> SRVLLALHDRAPQLKISDDRLTVVGEKGYSMVRASHGVRKGAWYFEITVDEMPPDTAARLGWSQPLGNLQAPLGYDKFSYSWRSKKGTKFHQSIGKHYSSGYGQGDVLGFYINLPEDISGRGSEIIFYKNGVNQGVAYKDIFEGVYFPAIS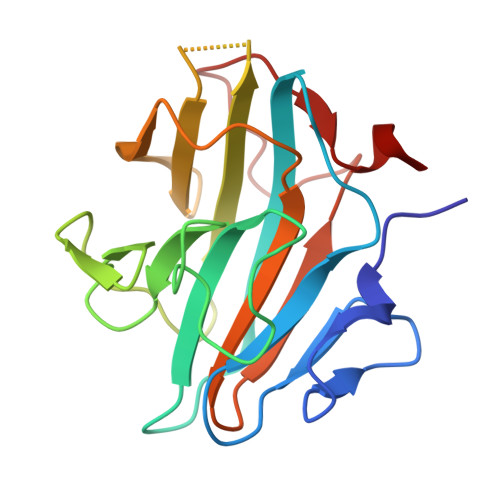LYKSCTVSINFGPCFKYPPKDLTYRPMSDMG>MGSSHHHHHHGSNQLTAYTLRLGDNCLVLSQRLGEWCGHAPELEIDLALANIGLDLLGQARNFLSYAAELAGEGDEDTLAFTRDERQFSNLLLVEQPNGNFADTIARQYFIDAWHVALFTRLMESRDPQLAAISAKAIKEARYHLRFSRGWLERLGNGTDVSGQKMQQAINKLWRFTAELFDADEIDIALSEEGIAVDPRTLRAAWEAEVFAGINEATLNVPQEQAYRTGGKKGLHTEHLGPMLAEMQYLQRVLPGQQW[8x];>MRSTQEERFEQRIAQETAIEPQDWMPDAYRKTLIRQIGQHAHSEIVGMLPEGNWITRAPTLRRKAILLAKVQDEAGHGLYLYSAAE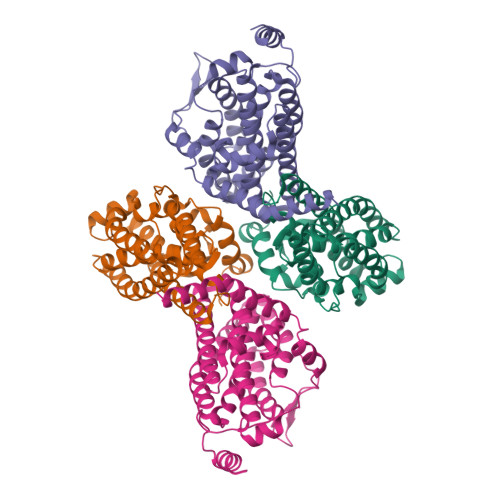TLGCAREDIYQKMLDGRMKYSSIFNYPTLSWADIGVIGWLVDGAAIVNQVALCRTSYGPYARAMVKICKEESFHQRQGFEACMALAQGSEAQKQMLQDAINRFWWPALMMFGPNDDNSPNSARSLTWKIKRFTNDELRQRFVDNTVPQVEMLGMTVPDPDLHFDTESGHYRFGEIDWQEFNEVINGRGICNQERLDAKRKAWEEGTWVREAALAHAQKQHARKVA[4x]>MASWSHPQFEKGAVTSLYKKAGFKDLTMLLDELKDMSFFNKGDICLIGCSTSEVIGEKIGTVGSMEVAETIFNALDVVSKETGVTFAFQGCEHINRAITIEKSQYNPLTMEEVSVVPDVHAGGSLATYAFQHMKDPIVVEHITVPCGIDIGQTLIGMHIKHVCVPVRTSVKQVGQAIVTIATSRPKKIGGERAKYQ[6x]

S. aureus YwlG is a 174-a.a.-long uncharacterized protein member of the UPF0340 family with a DUF436 domain of unknown function. Here, we describe a dual-function, hibernation factor hibernation-promoting factor (HPF) in pathogenic Staphylococcus aureus that dimerizes 70S ribosomes and represses YwlG-mediated glutamate dehydrogenase activity via a physical HPF–YwlG interaction. Conversely, YwlG binding to HPF reduces the formation of 100S ribosomes. Our data reveal the moonlighting role of YwlG in regulating the abundance of 100S ribosomes (via HPF) and the important role of YwlG in glutamate metabolism (via GDH activity).

We determined the X-ray crystallography structure of YwlG to 1.75-Å resolution and did not detect bound PLP or other ligands. The fold of YwlG is characterized by a central eight-stranded antiparallel β-sheet decorated with three large and three short α-helices with an unusual 12-residue-long carboxyl-terminal extension. The oligomeric state was determined by size-exclusion chromatography (SEC), in which YwlG was eluted with a size corresponding to a complex equivalent to a hexamer. Consistent with the SEC analysis, the asymmetric unit of the crystal was six protomers that made up two stacked trimers. The carboxyl-terminal extension appeared to interlock the oligomer. Analysis of the multimeric state of the protein showed that the hexamer was a stable composition, with a solvent-accessible surface area of 39,710 Å2 and a surface area upon hexamer formation of 12,540 Å2 (estimated G: −56.6 kcal/mol). We replaced the invariant residue C69 with a serine because C69 was oxidized in the crystals with unknown significance. The hexameric structure of S. aureus YwlG remotely resembles the structures of members of the catabolic, NAD-specific GDH family. First, YwlG is half of the typical size of a GDH and lacks the N-terminal catalytic domain and ligand binding sites. The inability to detect PLP or other cofactor binding in the YwlG protein crystal could be due to instability of YwlG in its PLP-bound form or the missing component(s), e.g., HPF, in the heterologous E. coli from which recombinant YwlG proteins were isolated.>MSAAPVLSITNASVVYPDGISTVTALDSANVEIFPGELVAIVGESGSGKSTLLSIAGFLQEPTSGTVTLHGAEGLDATSTRREHIGFVFQQPNLLGSLTAREQLLITDHLRGIKPRKDRADELLARVGLKGLGGRRVAQLSGGQRQRVNIARALMGNPQLLLADEPTSALDARLSKEIVELLRDVTKEFALATLMVTHDRSQLAYADRFVEMADGKALQTAKLWSHPQFEK[6x];>MFLGIRDIRAAAGRFALIASVVGLITLLIVMLTGLTQGLGKQNTSAIEALAPHSVVFTTAGGSSPEFTSSEISEQQAERWKDSTPLGVSQTRIESDQNANTTAVMGLPEGTPLPDSVGGFIEQGALLPAELADFLHVRAGDHITLGGATVTVAGTVKTENYSHTPVVWVDTATWQLVSHTKAVGTVLLLNQEPTIQPQDNEVVTDLKGAFQAMPAYKSERSSLLSMQAFLYIISALVTVAFLTVWTLQRTRDIAVLAALGASKRYLLIDALGQAAIILAAGVALGAGIGALLGWLIAGSVPFSLGWVSVLGPALGIWLLGLIGATIA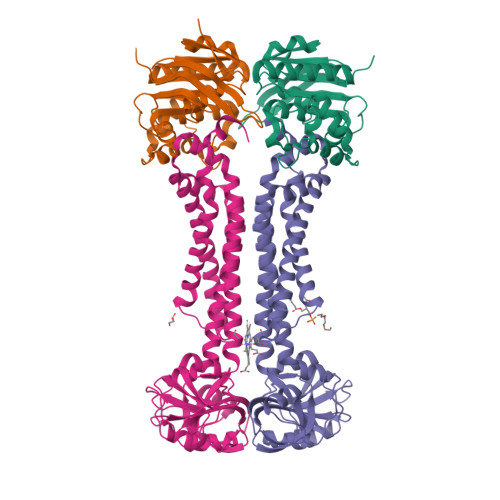VRNVTKVDPQIALGATA[6x]> MAFVSSGYNPEKPMENRISDIGPRHASDFFPPVIAKNKGQWLWHEICEPGILMHKAESGDEVYTVRCGGARLMSVGHIREICAIADKFCGGHLRFTTRNNIEFMVTTLDEAKKLKEYLNAQKFEGGSFKFPVGGTGAGITNIVHTQGWVHCHTPATDASGTVKVVLDELFEEFGQMRMPAQVRISMACCLNMCGAVHCSDIAIL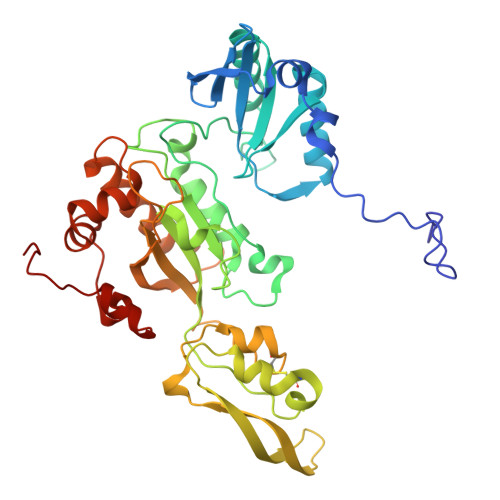GYHRKPPVIDHEWLDNLCEIPLAVAACPVGAIRPTKKEIVTEKGETKTVNTVAIKNERCMFCGNCYTMCPSLPLSDQTGDGLVIMAGGKVSNRISNPKFSKVVVAFIPNEPPRWPRLASVIRQIVEAYAADARKYERVGDWAERIGWERFFEKCELDFSIHMIDDFRDPAYYTWRQTTNFKF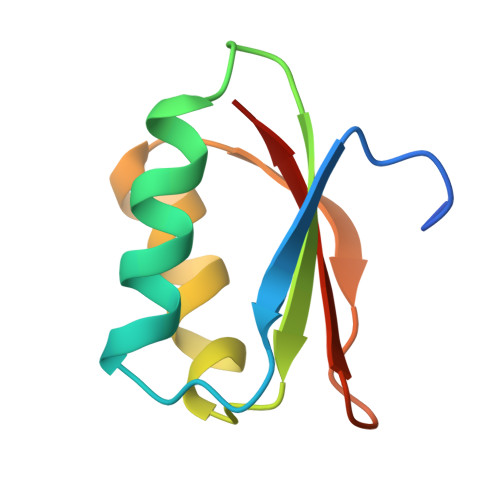> GSTDLFSSPDHTLDALGLRCPEPVMMVRKTVRNMQPGETLLIIADDPATTRDIPGFCTFMEHELVAKETDGLPYRYLIRKGG>MKGLVELGEKAPDFTLPNQDFEPVNLYEVLKRGRPAVLIFFPAAFSPVCTKELCTFRDKMAQLEKANAEVLAISVDSPWCLKKFKDENRLAFNLLSDYNR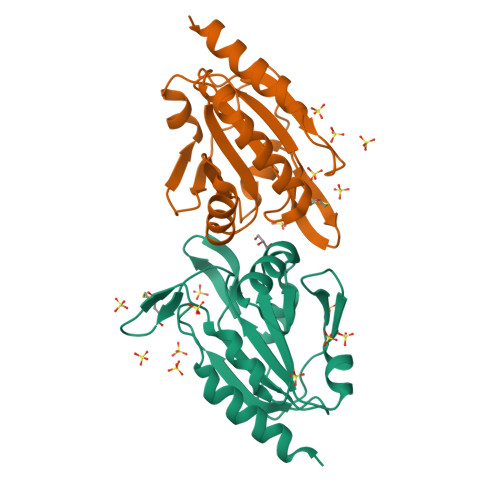EVIKLYNVYHEDLKGLKMVAKRAVFIVKPDGTVAYKWVTDNPLNEPDYDEVVREANKIAGELVA[4x]>QLTTESMPFNVAEGKEVLLLVHNLPQQLFGYSWYKGERADGNRQIVGYAIGTQQATPGPANSGRETIYPNA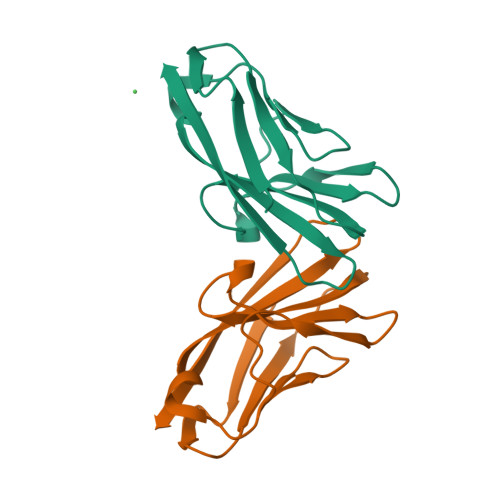SLLIQNVTQNDTGFYTLQVIKSDLVNEEATGQFHVY[4x]> MAHHHHHHVDDDDKSENLYFQGTANLTTSLLGDLLDDVTSIRHAVLQNRAAIDFLLL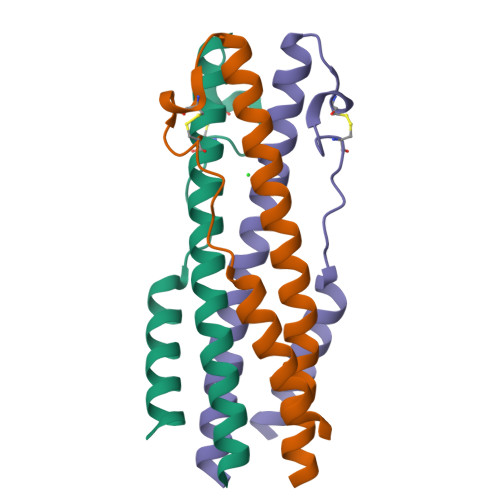AHGHGCEDVAGMCSFNLSDQSESIQKKFQLMKEHVNK>[2x]MHHHHHHSNNNTSIHDFDFSFICNYFKLLKRQGPGSPEATRKAVSFINELTDDAKIADIGCGTGGQTLFLADYVKGQITGIDLFPDFIEIFNENAVKANCADRVKGITGSMDNLPFQNEELDLIWSEGAIYNIGFERGMNEWSKYLKKGGFIAVSEASWFTSERPAEIEDFWMDAYPEISVIPTCIDKMERAGYTPTAHFILPENCWTEHYFAPQDEVRETFMKEHAGNKTAMDF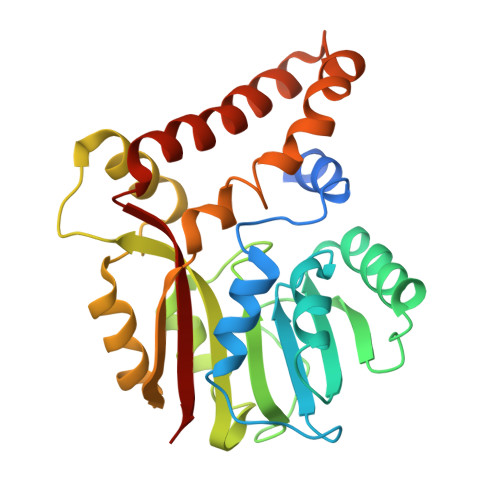MKGQQYERSLYSKYKDYYGYVFYIGQKR> ISADQVNQIIYNLHHDPFEILGCHLLEEGKNTKKWVVRAYLPKAEAAWVIRPTERKEDPMNSVHHPNFFECIIETPELNHYQLKVKEGEHEKVIYDPYAFSSPYLTDEDIYLFSEGNHHRIYEKLGAHVGEINGVKGVYFAVWAPNARNVSVIGDFNNWDGREHQMRKRNYTIWELFVPEIGSGTVYKYEIKNSEGHIYEKSDPYGFYREVRPNTASIVVDIDNIYQWHDEEWLEKRRNSDPLKQPVSVYEVHLGSWLHGSSAEKMPLLNGEADPVIVSEWNPGARFLSYYELAEKLIPYVKDMGYTHIELLPIAEHPFDGSWGYQVTGFYSPTSRFGRPEDFMYFVDKCHENGIGVILDWVPGHFPKDSHGLAYFDGTHLYEHADPRIGEHKEWGTLVFNYGRHEVRNFLVANVLFWFDKYHVDGIRVAAVASMLYRNYLRKEGEWIANEYGGDEHIEAVSFIREVNTLLFEYFPGILSIAEESTEWEKVSRPVYDGGLGFNLKWDMGWMHDMLDYFNIDPYFRQYHQNNVTFSMLYYYNENFMLALSHDEIVHGKSNMLGKMPGDEWQKYANVRALFTYMYTHPGKKTMFMSMEFGQWSEWNVWGDLEWHLLQYEPHQQLKQFFTDLNALYQQEPALYTHDFEYHGFEWIDCNDNTHSVVSFLRRSDDPNDSLVVVCNFTPQPHS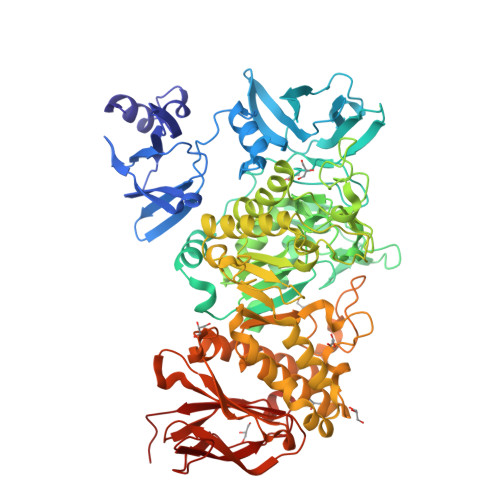HYRIGVPEAGYYVELFNSDAKQYGGSNMGNLGGKWADEWSFHNKPYSLDLCLPPLAVLILKLDPTKVP> MTITLIEPVQQRTGIYPSSDLKVEDGYPSSDTFQIIQTQDGRGA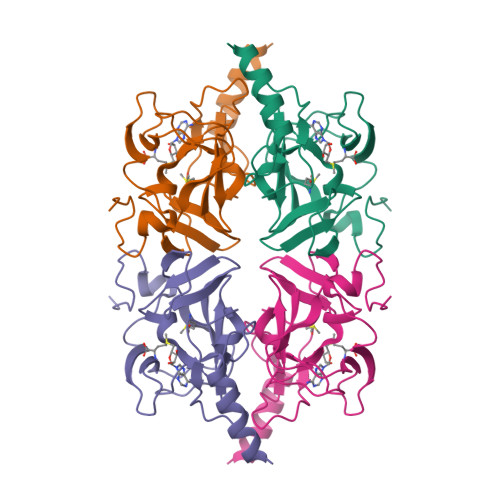GVRVLKTFARGRRMARVSGQITAFCRLHTLQINAHTHLYDPHFSGLLLHSCVPNVRLDMAGFELWSLRDIAAGEMLTMDYASTEDVLMRQFECHCGAPNCRRWITGAKELPNDIGQALLAGLRAAALALEHHHHHH> GDPVEDIIHDALGNTARRAISSATNVESAANTTPSSHRLETGRVPALQAAETGATSNATDENMIETRCVVNRNGVLETTINHFFSRSGLVGVVNLTDGGTDTTGYATWDIDIMGFVQLRRKCEMFTYMRFNAEFTFVTTTENGGARPYMLQYMYVPPGAPKPTGRDAFQWQTATNPSVFVKLTDPPAQVSVPFMSPASAYQWFYDGYPTFGQHPETSNTTYGLCPNNMMGTFAVRVVSREASQLKLQTRVYMKLKHVRAWVPRPIRSQPYLLKNFPNYDSSKITNSARDRSSIKQANM;> MGAQVSTQKSGSHETGNVATGGSTINFTNINYYKDSYAASATRQDFTQDPKKFTQPVLDSIRELSAPLNSPSVEACGYSDRVAQLTVGNSSITTQEAANIVLAYGEWPEYCPDTDATAVDKPTRPDVSVNRFYTLDSKMWQENSTGWYWKFPDVLNKTGVFGQNAQFHYLYRSGFCLHVQCNASKFHQGALLVAVIPEFVIAGRGSNTKPNEAPHPGFTTTFPGTTGATFY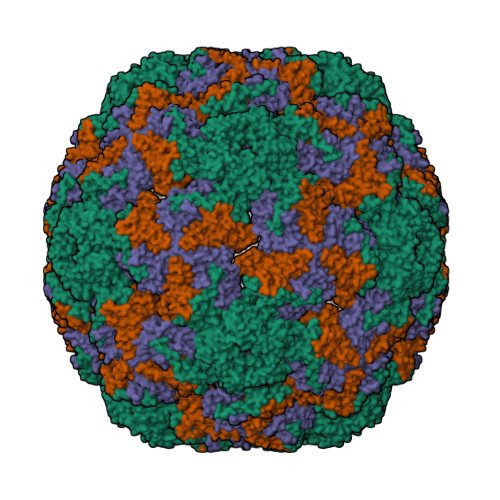DPYVLDSGVPLSQALIYPHQWINLRTNNCATVIVPYINAVPFDSAINHSNFGLIVIPVSPLKYSSGATTAIPITITIAPLNSEFGGLRQAVSQ;> GIPAELRPGTNQFLTTDDGTAAPILPGFTPTPTIHIPGEVHSLLELCRVETILEVNNTTEATGLTRLLIPVSSQNKADELCAAFMVDPGRIGPWQSTLVGQICRYYTQWSGSLKVTFMFTGSFMATGKMLVAYSPPGSAQPANRETAMLGTHVIWDFGLQSSVSLVIPWISNTHFRTAKTGGNYDYYTAGVVTLWYQTNYVVPPETPGEAYIIAMGAAQDNFTLKICKDTDEVTQQAVLQ>MGSLMYLLRLVCFLTLLGVTAALFIFAVDLAVHGLEELRMKISRLAGRFAGYILYVVSGVALCLLSTFWCAVLSTEAEGSGLPQMKSILSGFYDKMRSALELRVLFAKALGLICAIGGGLPVGWEGPNVHIACIIAHQFYRLGVFKELCTDRALRLQTLAAACAVGLASSFGAPLGGVLYSIETIASFYLVQAFWKGVLSALSGAIVYELLYTTPLVEAFEGTNFDASDVSRTQTLLYAILGALMGVLGALFIRCVRSIYELRMRHYPGTNRYFLVGVVALFASALQYPFRLFALDPRATINDLFKAVPLYQTDHFGWTELILMPIIKFILVALSIGLPLPAGVFVPSFLIGAGFGRLYGELMRVVFGNAIVPG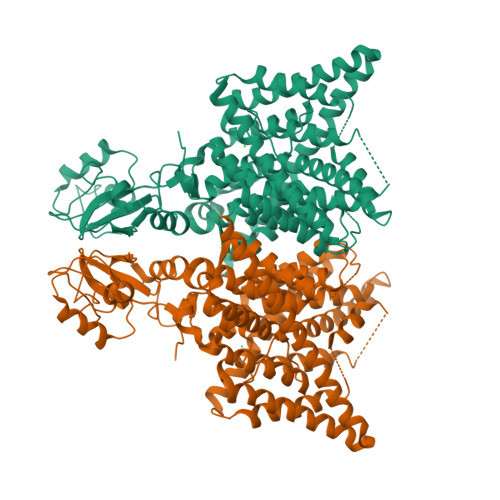SYAVVGAAAFTAGVTRALSCAVIIFEVTGQIRHLVPVLISVLLAVIVGNAFNRSLYETLVLMKHLPYMPILRRDRSPEMTAREIMHPIEGEPHLFPDSEPQHIKGILEKFPNRLVFPVIDANGYLLGAISRKEIVDRLQHVLEDVPEPIAGHRTLVLLDAADLSENIEGLVDETPSGEHSSKGKRTATVLEPTSSLVVPCDVSPIVVTSYSLVRQLHFLFVMLMPSMIYVTERGKLVGIVEREDVAYGYSNSLEVLFQ[4x]> MVYIALFALGAALVTLFFYLILNPRVLTTEGETFDL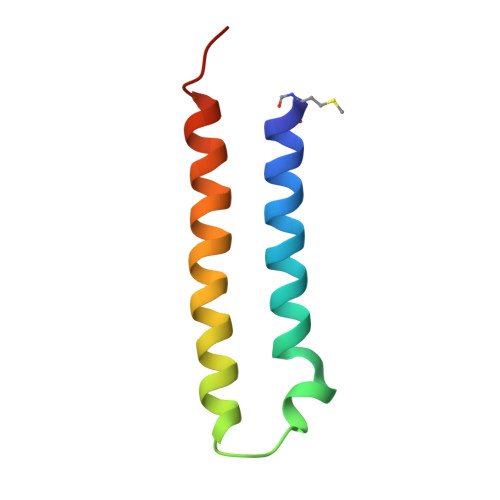RFVLFMLLLILLAAGTVALMLLIGKAHHLL>[4x]MAHHHHHHMSSAESNIPEQFRIRRDKRARLLAEGYDPYPVAIERTHTLAEIRATYADLPTDSATEDIVGVAGRVVFARNTGKLCFATLQDGDGTQLQAMISLDEVGRESLDRWKADVDIGDVVYVHGTVI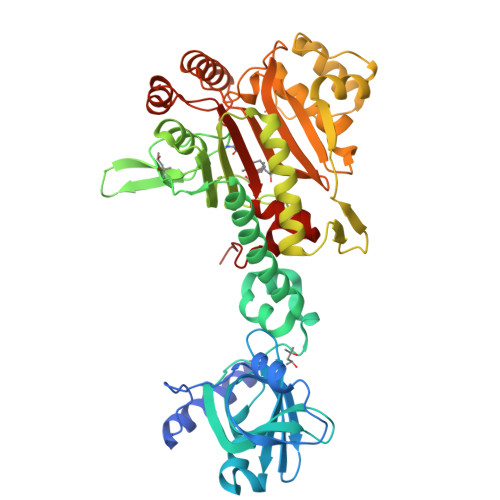SSRRGELSVLADSWRMAAKALRPLPVAHKEMSEESRVRQRYVDLIVRPQAREVARQRIAVIRAVRNALERRGFLEVETPMLQTLAGGAAARPFVTHSNALDIDLYLRIAPELFLKRCIVGGFDRVFELNRVFRNEGSDSTHSPEFSMLETYQTYGTYDDSALITRELIQEVADEAIGTRQLSMPDGSVYDIDGEWATMEMYSSLSEALGEQITPETTVARLRDIASGLDVEIDNSVFGHGKLVEELWEHAVGNKLTAPTFVKDFPVETTPLTRQHRSIPGVTEKWDLYVRGVELATGYSELNDPVVQRDRFADQARAAAAGDDEAMQLDEDFLTALEYGMPPCTGTGMGIDRLLMCLTGLSIRETVLFPIVRPHSN> MQAAKQLSQNFLLDLRLTDKIVRKAGNLTNAYVYEVGPGPGGITRSILNADVAELLVVEKDTRFIPGLQMLSDAAPGKLRIVHGDVLTFKVEKAFSESLKRPWEDDPPNVHIIGNLPFSVSTPLIIKWLENISCRDGPFVYGRTQMTLTFQKEVAERL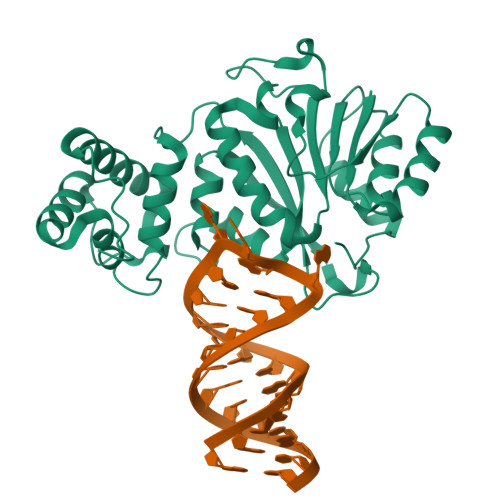AANTGSKQRSRLSVMAQYLCNVRHIFTIPGQAFVPKPEVDVGVVHFTPLIQPKIEQPFKLVEKVVQNVFQFRRKYCHRGLRMLFPEAQRLESTGRLLELADIDPTLRPRQLSISHFKSLCDVYRKMCDEDPQLFAYNFREELKRRKSKNEEKEEDDAENYRL6-chloro-4-methyl-1H-quinolin-2-one | C10 H8 Cl N O | 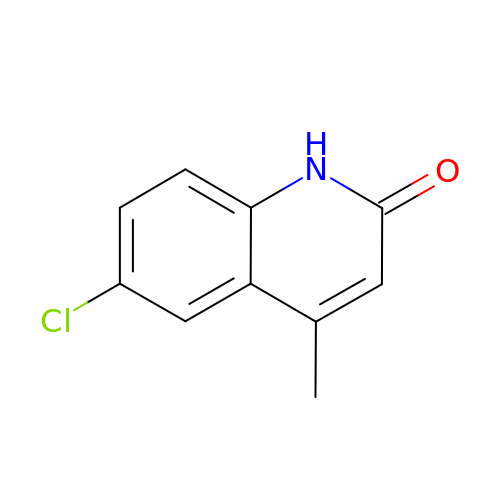VQMIYHVFVPSLGB-UHFFFAOYSA-N>[2x]HHHHHHHHGGLVPRGSHGGSMTDRLKGKVAIVTGGTLGIGLAIADKFVEEGAKVVITGRHADVGEKAAKSIGGTDVIRFVQHDA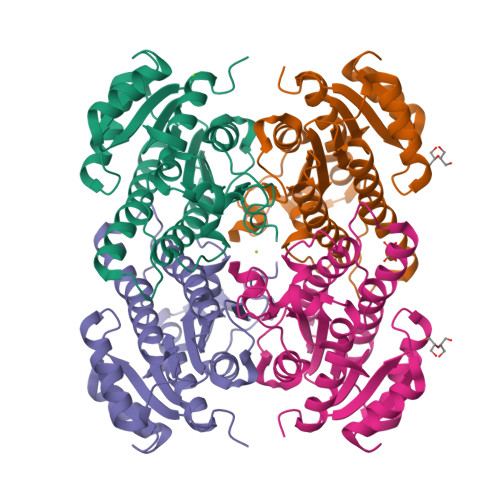SDEAGWTKLFDTTEEAFGPVTTVVNNAGIFVSKSVEDTTTEEWRKLLSVNLDGVFFGTRLGIQRMKNKGLGASIINMSSIEGFVGDPTLGAYNASKGAVRIMSKSAALDCALKDYDVRVNTVHPGYIKTPLVDDLEGAEEMMSQRTKTPMGHIGEPNDIAWICVYLASDESKFATGAEFVVDGGYTAQ> AEQSSSEIKIVRDEYGMPHIYANDTWHLFYGYGYVVAQDRLFQMEMARRSTQGTVAEVLGKDFVKFDKDIRRNYWPDAIRAQIAALSPEDMSILQGYADGMNAWIDKVNTNPETLLPKQFNTFGFTPKRWEPFDVAMIFVGTM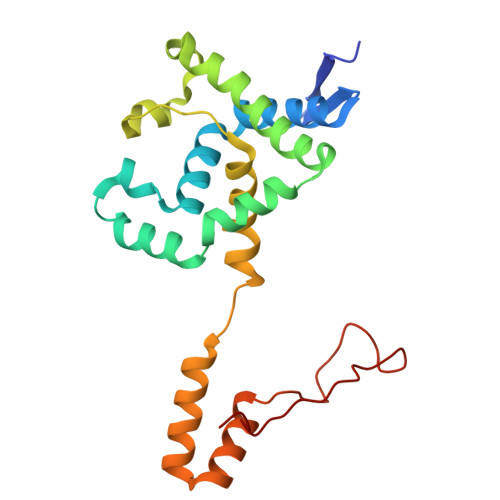ANRYSDSTSEIDNLALLTALKDKYGVSQGMAVFNQLKWLVNPSAPTTIAVQESNYPLKFNQQNSQT>MNLIPTVIETTNRGERAYDIYSRLLKDRIIMLGSQIDDNVANSIVSQLLFLQAQDSEKDIYLYINSPGGSVTAGFAIYDTIQHIKPDVQTICIGMAASMGSFLLAAGAKGKRFALPNAEVMIHQPLGGAQGQATEIEIAANHILKTREKLNRILSERTGQSIEKIQQDTDRDNFLTAAEAKEYGLIDEVMEPEHHHHHH[14x]

Bacterial caseinolytic protease P subunit (ClpP) is important and vital for cell survival and infectivity. The caseinolytic protease P (ClpP) subunit is a compartmentalized structure with two stacked heptameric rings that form a central chamber containing 14 identical catalytic sites sequestered by two protective axial pores. In any case, even the degradation of small oligopeptides depends on some structural factors, and the most important one is the orientation and positioning of the catalytic triads formed by Ser98, His123, and Asp17224. The protein’s mode of action corresponds to that of a chymotrypsin-like protease, and it is described in two main steps: acylation and deacylation.

Aiming to explore and explain this paradoxical effect, we solved and refined the crystal structure of native ClpP from Staphylococcus epidermidis (Se), an opportunistic pathogen involved in nosocomial infections, as well as ClpP in complex with ixazomib at 1.90 Å and 2.33 Å resolution, respectively. The crystal structures of native SeClpP and SeClpP-ixazomib complex were refined to 1.90 Å and 2.33 Å, respectively. The superimposition of both tetradecameric structures displays that the complex is slightly more extended than the apo SeClpP, and the Cα RMSD is 1.63 Å for 1451 atoms. When SeClpP monomers from both structures are compared, the Cα RMSD is 0.12 Å for 164 atoms. In both cases, the monomers are composed of a common structure consisting of the following main parts: E-helix with a Gly-rich region, catalytic site, head domain, oligomerization sensor, and N-terminal loop. Despite the similarity between the overall structures and the high homology between amino acid sequences of ClpPs from different species, a closer look into the monomers exhibits a difference in the Gly-rich region. The structure in this region seems to be more ordered when ixazomib is present. Figure 2c shows that the apo SeClpP has a more disordered Gly-rich region with an unstructured loop and two small antiparallel beta-strands formed by two subunits from opposing heptameric rings. A comparative analysis with the native SeClpP, the SeClpP-ixazomib complex, and SaClpP Y63A29 structures revealed that the Asn42 side chain in the complex, as well as in the mutant, is shifted to the “down” position (the hydroxyl group is approx. 5 Å distant from Tyr21). In the native protein, the residue is found in the “up” position, as expected.> MARQNLKSTDRAVQQMLDKAKREGIQTVWDRYEAMKPQCGFGETGLCCRHCLQGPCRINPFGDEPKVGICGATAEVIVARGLDRSIAAGAAGHSGHAKHLAHT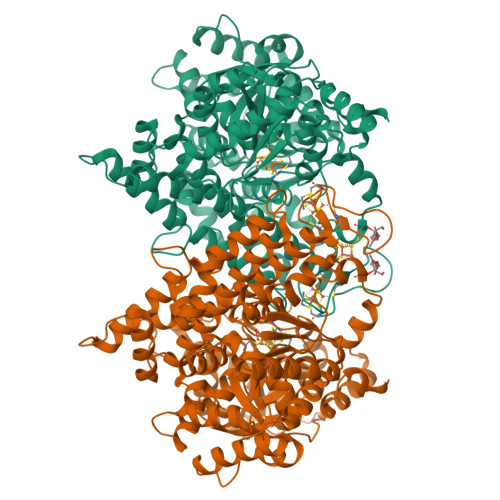LKKAVQGKAASYMIKDRTKLHSIAKRLGIPTEGQKDEDIALEVAKAALADFHEKDTPVLWVTTVLPPSRVKVLSAHGLIPAGIDHEIAEIMHRTSMGCDADAQNLLLGGLRCSLADLAGCYMGTDLADILFGTPAPVVTESNLGVLKADAVNVAVHGHNPVLSDIIVSVSKEMENEARAAGATGINVVGICCTGNEVLMRHGIPACTHSVSQEMAMITGALDAMILDYQCIQPSVATIAECTGTTVITTMEMSKITGATHVNFAEEAAVENAKQILRLAIDTFKRRKGKPVEIPNIKTKVVAGFSTEAIINALSKLNANDPLKPLIDNVVNGNIRGVCLFAGCNNVKVPQDQNFTTIARKLLKQNVLVVATGCGAGALMRHGFMDPANVDELCGDGLKAVLTAIGEANGLGGPLPPVLHMGSCVDNSRAVALVAALANRLGVDLDRLPVVASAAEAMHEAAVAIGTWAVTIGLPTHIGVLPPITGSLPVTQILTSSVKDITGGYFIVELDPETAADKLLAAINERRAGLGLPW(2R,3R,4S,5S,6R)-2,3,4,5-tetrahydroxy-6-(hydroxymethyl)oxane-2-carboxamide | C7 H13 N O7 | 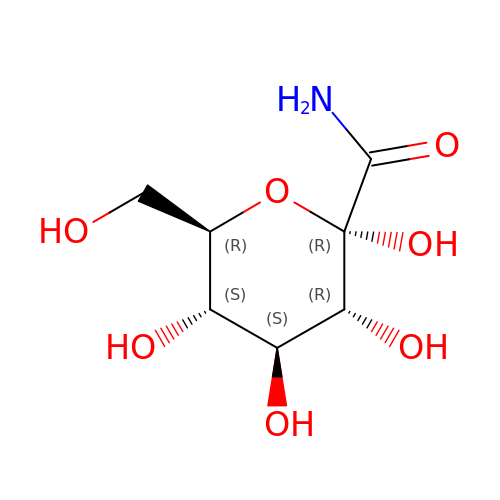DTZYCNDAJQDPQC-UHKLXPPTSA-N> CAGCATCGCCTGACACA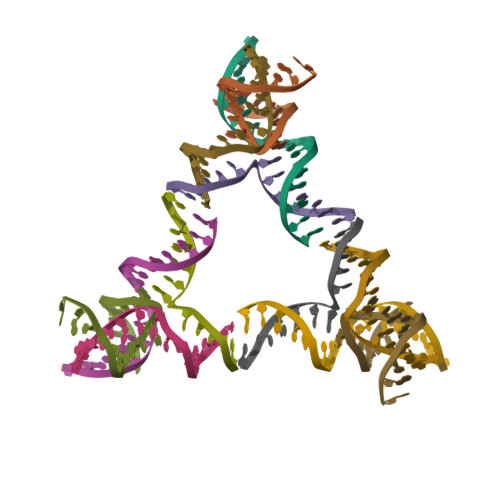;> CGTGGACATGCGAG;> TGCTCGCATGTGGCGATGC;> TGTGTCACCACG>AKKIGLFYGTQTGKTESVAEIIRDEFGNDVVTLHDVSQAEVTDLNDYQYLIIGCPTWNIGELQSDWEGLYSELDDVDFNGKLVAYFGTGDQAGYADNFQDAIGILEEKISQRGGKTVGYWSTDGYDFNDSKALRNGKFVGLALD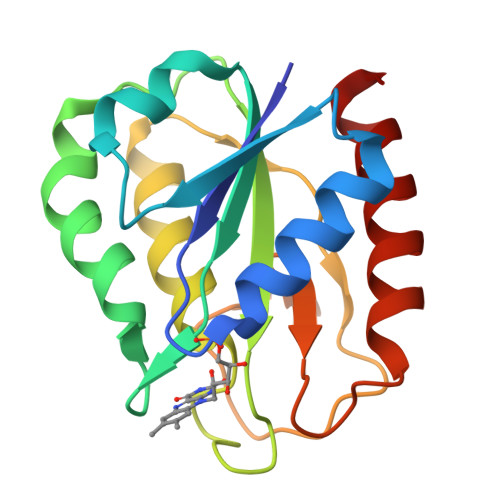EDNQSDLTDDRIKSWVAQLKSEFGL[2x]> MTATPQGQIIHHRNFQSLYNNSWVCSLNVIKSRDGNNYSALEDITSDNQAFNNILEGIDIIECENLLKEMNVQKIPESSLFTNIKEALQAEVFNSTVEDNFESFISYELQNHGPLMLIRPSLGSECLHAECIVGYDSEVKKVLIYDSMNTSPEWQSNIDVYDKLTLAFNDKYKNEDCSICGLYYDGVYEPKLEHHHHHH

In S. Typhimurium, which infects a broad range of hosts, another effector, GtgE, plays an essential role in virulence. GtgE is encoded within the Gifsy-2 lambdoid prophage. GtgE is a cysteine protease and contains a Cys-His-Asp catalytic triad. The critical base was identified as His151, the nucleophile as Cys45 and the third residue as Asp169.

Based on this information we have prepared two deletion mutants GtgE(17–214, Δ33–40, C45S) and GtgE(17–214, Δ59–68, C45S). Expression and purification of these mutants resulted in high yields of both constructs, suggesting that the mutations did not disrupt the structure. Both mutants were screened for crystallization, and the GtgE(17–214, Δ33–40, C45S) mutant produced large crystals diffracting to high resolution. Our structure of GtgE shows that the enzyme has a papain-like fold, composed of a slightly bent seven-stranded ß-sheet with two ¶-helices on the convex side and three on the concave side. Asp169 is located at the end of strand ß5 and Ser45 (cysteine in the wild type enzyme) is near the N-terminus of helix α1. Thus the N-terminal ~20 residues complete the papain fold of the neighboring molecule, which in turn donates this segment back to the first molecule. Through this swap of their N-termini the two molecules form a tight dimer in the crystal. Since the molecular weight determined by the SEC-MALS of 25.5 kDa indicated that the protein is predominantly a monomer in solution, this swap is likely the crystallization artefact. Comparison with papain and other papain-like enzymes suggests that helix α1 in GtgE is longer by one turn on the N-terminal end and starts four residues earlier. This additional turn of the helix enters the area corresponding to the classic substrate-binding site of papain-like enzymes and partially blocks it. We conclude that the function of GtgE in vivo as a proteolytic enzyme is likely dependent on other factor(s), such as a protein partner or interactions with the SCV membrane, which cause a realignment of the catalytic triad to its active conformation stimulating GtgE activity in vivo.>[2x]HMTAIKTRPVHGYSKFLSTGSARGSRVVTNKEMCTLIDSTPEWIEQRTGITERRWATNSETVASMGTTAA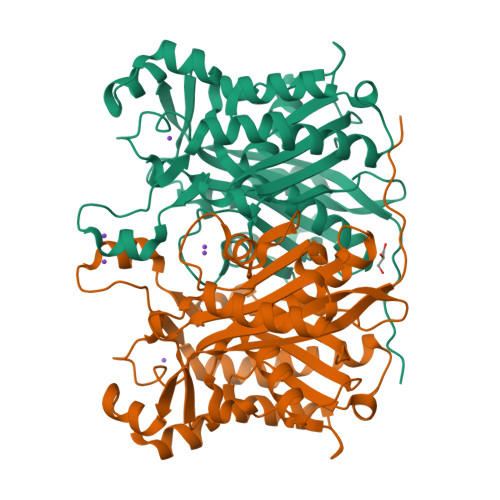RTALERSGLEASQIDAIIVATVSHHRPSPSLAAYIARELGLGDAAAFDLNGAAAGFCYSTALADSMIRTGSANYVLVIGVEKLSEMTNLDDRSTAFLFSDGAGAAIIGASDEPGIGPVVWGSRSDQLKTIELEDWPTASADPNKIHPLIRMEGRAVFKWAMTDVAKRAAEAIAEAGITPADLDVFIPHQANDRITDVVSRHLKLPESVTVCHDIADMGNTSAASVPIAIDRMLQRGQAHSGDLALIIGFGAGLVYAGQVIRLP>MIKLCIAGKNNIAVNSLEYILKNHFKPDQVAVIPNKNDFGVDSWQKSLLHYAFNNHIKVITLEEAYELKQIIFFSLEFDRIVKVEKFKSDKLFNMHFSALPKYKGVFTSITPILNNEVESGVTLHCIDNGIDTGNIIDQYIFPININDTARDLYFNYLSYGEYLFKKNIQRIINNTYENFKQNNISSSYFSRQDININHKINFKKTSFEIHNQIRAFIFKEYQLPSINKTKIIKSTLTNEFIGYNMFEEFEEYFMISGIDGFKIIAQKYNAELEHHHH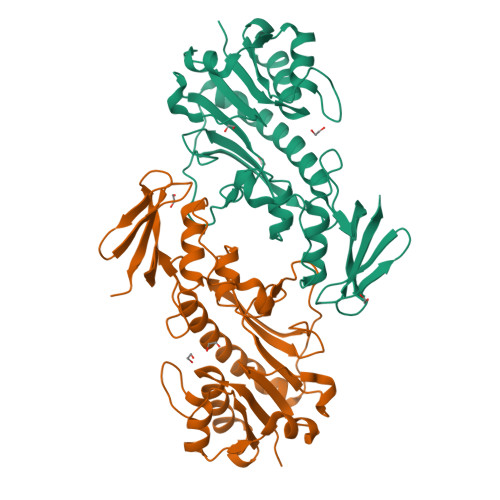HH[2x]5-[(4-methoxynaphthalen-1-yl)methyl]-1-[2-[(2-methyl-1-oxidanyl-propan-2-yl)amino]ethyl]-~{N}-(naphthalen-1-ylmethyl)-6,7-dihydro-4~{H}-pyrazolo[4,3-c]pyridine-3-carboxamide 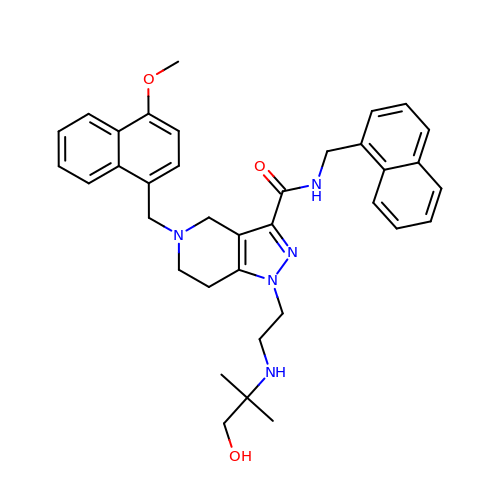| C36 H41 N5 O3 | MZJWSMMILGDGIP-UHFFFAOYSA-N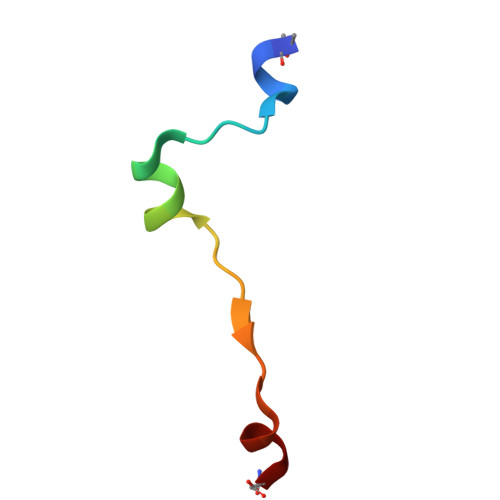> ADSESEFENVANAGSMEQFETIDHKDLN> GDVEEAIDRAVARVADTMPTGPRNTESVPALTAVETGHTSQVVPGDTMQTRHVKNYHSRTESSIENFLCRAACVYIATYKSAGGTPTERYASWRINTRQMVQLRRKFELFTYLRFDMEITFVITSTQDPGTQLAQDMPVLTHQIMYIPPGGPVPNSATDFAWQSSTNPSIFWTEGCAPARMSVPFISIGNAYSNFYDGWSHFTQEGVYGFNSLNNMGHIYVRHVNEQSLGVSTSTLRVYFKPKHVRAWVPRPPRLSPYVKSSNVNFKPTAVTTERKDINDVGTLRPVGYTNH;> GAQVSTQKTGAHETSLTASGNSTIHYTNINYYKDAASNSANRQDFTQDPSKFTEP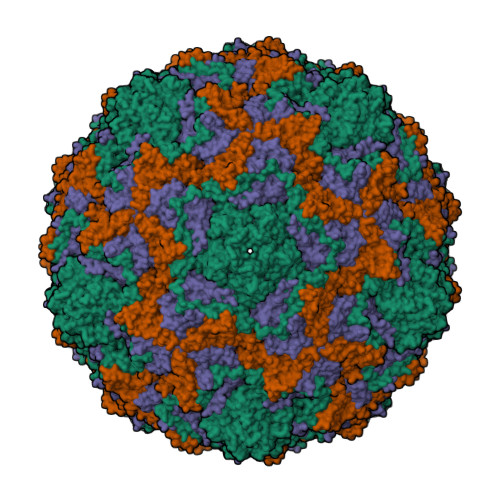MKDVMIKSLPALNSPTVEECGFSDRVRSITLGNSTITTQECANVVVGYGVWPSYLQDNEATAEDQPTQPDVATCRFYTLDSIQWQKESDGWWWKFPEALKNMGLFGQNMEYHYLGRSGYTIHVQCNASKFHQGCLLVVCVPEAEMGCSDVEREVVAASLSSEDTAKSFSRTESNGQHTVQTVVYNAGMGVGVGNLTIFPHQWINLRTNNSATIVMPYINSVPMDNMFRHYNFTLMIIPFAKLEYTEQASNYVPITVTVAPMCAEYNGLRLASHQ;> GLPTMLTPGSNQFLTSDDFQSPSAMPQFDVTPEMKIPGEVHNLMEIAEVDSVVPVNNTKENINSMEAYRIPVTGGDQLHTQVFGFQMQPGLNSVFKRTLLGEILNYYAHWSGSVKLTFVFCGSAMATGKFLLAYSPPGASPPQNRKQAMLGTHVIWDVGLQSSCVLCIPWISQTHYRLVQQDEYTSAGYVTCWYQTGLIVPPGAPPSCTILCFASACNDFSVRNLRDTPFIEQTQLLQ>[10x]MNVSEALKGALPNFIPGL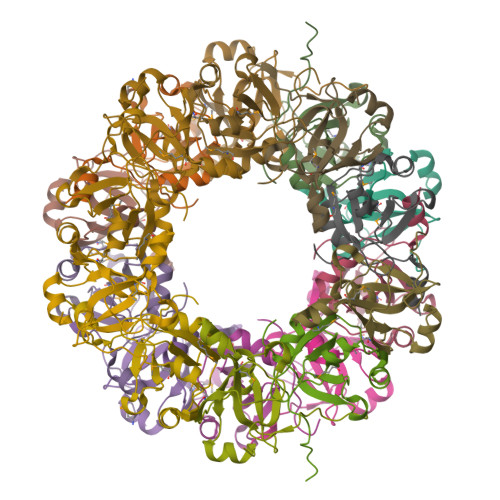GTLYVDPSTLPEGPFLAYDRAGNLVKVVFMVPLKKLNESHKYVDIGTKTLRALGITRIDHVNMIPSGPHPGVSEPHYHIELVLVSVDQERKVLEGEPY> NTALAEMPKRKFTIDDFDIGRPLGKGKFGNVYLAREKQNKFIMALKVLFKSQLEKEGVEHQLRREIEIQSHLRHPNILRMYN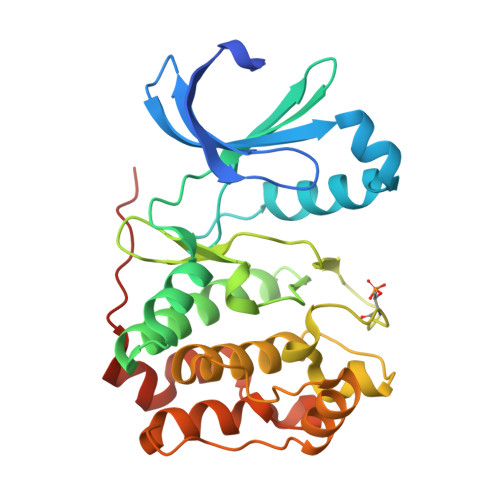YFHDRKRIYLMLEFAPRGELYKELQKHGRFDEQRSATFMEELADALHYCHERKVIHRDIKPENLLMGYKGELKIADFGWSVHAPSLRRRTMCGTLDYLPPEMIEGKTHDEKVDLWCAGVLCYEFLVGMPPFDSPSHTETHRRIVNVDLKFPPFLSDGSKDLISKLLRYHPPQRLPLKGVMEHPWVKANSRRVLPPVYQSTQSK> MSGLPPPPPGFEEDSDLALPPPPPPPPGYEIEELDNPMVPSSVNEDTFLPPPPPPPSNFEINAEEIVDFTLPPPPPPPGLDELETKAEKKVELHGKRKLDIGKDTFVTRKSRKRAKKMTKKAKRSNLYTPKAEMPPEHLRKIINTHSDMASKMYNTDKKAFLGALKYLPHAILKLLENMPHPWEQAKEVKVLYHTSGAITFVNETPRVIEPVYTAQWSATWIAMRREKRDRTHFKRMRFPPFDDDEPPLSYEQHIENIEPLDPINLPLDSQDDEYVKDWLYDSRPLEEDSKKVNGTSYKKWSFDLPEMSNLYRLSTPLRDEVTDKNYYYLFDKKSFFNGKALNNAIPGGPKFEPLYPREEEEDYNEFNSIDRVIFRVPIRSEYKVAFPHLYNSRPRSVRIPWYNNPVSCIIQNDEEYDTPALFFDPSLNPIPHFIDNNSSLNVSNTKENGDFTLPEDFAPLLAEEEELILPNTKDAMSLYHSPFPFNRTKGKMVRAQDVALAKKWFLQHPDEEYPVKVKVSYQKLLKNYVLNELHPTLPTNHNKTKLLKSLKNTKYFQQTTIDWVEAGLQLCRQGHNMLNLLIHRKGLTYLHLDYNFNLKPTKTLTTKERKKSRLGNSFHLMREL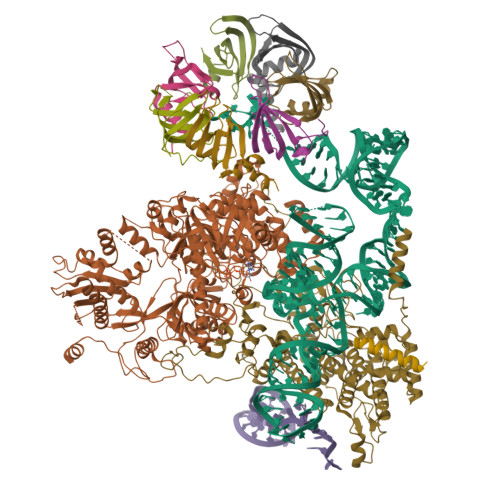LKMMKLIVDTHVQFRLGNVDAFQLADGIHYILNHIGQLTGIYRYKYKVMHQIRACKDLKHIIYYKFNKNLGKGPGCGFWQPAWRVWLNFLRGTIPLLERYIGNLITRQFE;> MEGDDLFDEFGNLIGVDPFDSDEEESVLDEQEQYQTNTFEGSGNNNEIESRQLTSLGSKKELGISLEHPYGKEVEVLMETKNTQSPQTPLVEPVTERTKLQEHTIFTQLKKNIPKTRYNRDYMLSMANIPERIINVGVIGPLHSGKTSLMDLLVIDSHKRIPDMSKNVELGWKPLRYLDNLKQEIDRGLSIKLNGSTLLCTDLESKSRMINFLDAPGHVNFMDETAVALAASDLVLIVIDVVEGVTFVVEQLIKQSIKNNVAMCFVINKLDRLILDLKLPPMDAYLKLNHIIANINSFTKGNVFSPIDNNIIFASTKLGFTFTIKEFVSYYYAHSIPSSKIDDFTTRLWGSVYYHKGNFRTKPFENVEKYPTFVEFILIPLYKIFSYALSMEKDKLKNLLRSNFRVNLSQEALQYDPQPFLKHVLQLIFRQQTGLVDAITRCYQPFELFDNKTAHLSIPGKSTPEGTLWAHVLKTVDYGGAEWSLVRIYSGLLKRGDTVRILDTSQSESRQKRQLHDISKTETSNEDEDSKTETPSCEVEEIGLLGGRYVYPVHEAHKGQIVLIKGISSAYIKSATLYSVKSKEDMKQLKFFKPLDYITEAVFKIVLQPLLPRELPKLLDALNKISKYYPGVIIKVEESGEHVILGNGELYMDCLLYDLRASYAKIEIKISDPLTVFSESCSNESFASIPVSNSISRLGEENLPGLSISVAAEPMDSKMIQDLSRNTLGKGQNCLDIDGIMDNPRKLSKILRTEYGWDSLASRNVWSFYNGNVLINDTLPDEISPELLSKYKEQIIQGFYWAVKEGPLAEEPIYGVQYKLLSISVPSDVNIDVMKSQIIPLMKKACYVGLLTAIPILLEPIYEVDITVHAPLLPIVEELMKKRRGSRIYKTIKVAGTPLLEVRGQVPVIESAGFETDLRLSTNGLGMCQLYFWHKIWRKVPGDVLDKDAFIPKLKPAPINSLSRDFVMKTRRRKGISTGGFMSNDGPTLEKYISAELYAQLRENGLVP;> MSKIQVAHSSRLANLIDYKLRVLTQDGRVYIGQLMAFDKHMNLVLNECIEERVPKTQLDKLRPRKDSKDGTTLNIKVEKRVLGLTILRGEQILSTVVEDKPLLSKKERLVRDKKEKKQAQKQTKLRKEKEKKPGKIAKPNTANAKHTSSNSREIAQPSSSRYNGGNDNIGANRSRFNNEAPPQTRKFQPPPGFKRK;> MTMNGIPVKLLNEAQGHIVSLELTTGATYRGKLVESEDSMNVQLRDVIATEPQGAVTHMDQIFVRGSQIKFIVVPDLLKNAPLFKKNSSRPMPPIRGPKRR;> MSNKVKTKAMVPPINCIFNFLQQQTPVTIWLFEQIGIRIKGKIVGFDEFMNVVIDEAVEIPVNSADGKEDVEKGTPLGKILLKGDNITLITSAD;> MSESSDISAMQPVNPKPFLKGLVNHRVGVKLKFNSTEYRGTLVSTDNYFNLQLNEAEEFVAGVSHGTLGEIFIRCNNVLYIRELPN;> MVSTPELKKYMDKKILLNINGSRKVAGILRGYDIFLNVVLDDAMEINGEDPANNHQLGLQTVIRGNSIISLEALDAI;> MKLVNFLKKLRNEQVTIELKNGTTVWGTLQSVSPQMNAILTDVKLTLPQPRLNKLNSNGIAMASLYLTGGQQPTASDNIASLQYINIRGNTIRQIILPDSLNLDSLLVDQKQLNSLRRSGQIANDPSKKRRRDFGAPANKRPRRGL;> MSSQIIDRPKHELSRAELEELEEFEFKHGPMSLINDAMVTRTPVIISLRNNHKIIARVKAFDRHCNMVLENVKELWTEKKGKNVINRERFISKLFLRGDSVIVVLKTPVE> MGNDISLIALLAFSTLLPFIIASGT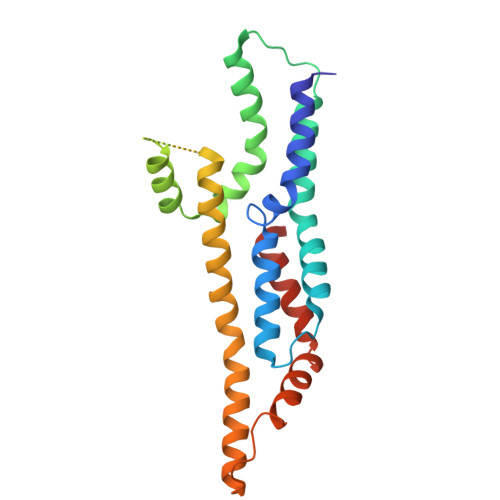CFVKFSIVFVMVRNALGLQQIPSNMTLNGVALLLSMFVMWPIMHDAYVYFEDEDVTFNDISSLSKHVDEGLDGYRDYLIKYSDRELVQFFENAQLKRQYGEETETVKRDKDEIEKPSIFALLPAYALSEIKSAFKIGFYLYLPFVVVDLVVSSVLLALGMMMMSPVTISTPIKLVLFVALDGWTLLSKGLILQYMDIAT>SMPSETPQAEVGPTGCPHRSGPHSAKGSLEKGSPEDKEAKEPLWIRPDAPSRCTWQLGRPASESPHHHTAPAKSPKILPDILKKIGDTPMVRINKIGKKFGLKCELLAKCEFFNAGGSVKDRISLRMIEDAERDGTLKPGDTIIEPTSGNTGIGLALAAAVRGYRCIIVMPEKMSSEKVDVLRALGAEIVRTPTNARFDSPESHVGVAWRLKNEIPNSHILDQYRNASNPLAHYDTTADEILQQCDGKLDMLVASVGTGGTITGIARKLKEKCPGCRIIGVDPEGSILAEPEELNQTEQTTYEVEGIGYDFIPTVLDRTVVDKWFKSNDEEAFTFARMLIAQEGLLCGGSAGSTVAVAVKAAQELQEGQRCVVILPDSVRNYMTKFLSDRWMLQKGFLKEEDLTEKKPWWWHLRVQELGLSAPLTVLPTITCGHTIEILREKGFDQAPVVDEAGVILGMVTLGNMLSSLLAGKVQPSDQVGKVIYKQFKQIRLTDTLGRLSHILEMDHFALVVHEQIQYHSTGKSSQRQMVFGVVTAIDLLNFVAAQERDQK[8x]

Cystathionine beta-synthase (CBS) is an essential metabolic enzyme across all domains of life for the production of glutathione, cysteine, and hydrogen sulfide. Human CBS adopts a unique multi-domain structure: an N-terminal haem binding domain (residues 38–74), a central PLP-dependent catalytic domain (CD, residues 75–382), and a C-terminal regulatory domain (RD, residues 411–551)5,11,12. The RD adopts the evolutionarily conserved Bateman module, consisting of two tandem CBS motifs (CBS-1 and CBS-2) and a surface-exposed loop (residues 516–525) extending from a CBS-2 motif. Here we show using cryo-electron microscopy that full-length human CBS in the basal and SAM-bound activated states polymerises as filaments mediated by a conserved regulatory domain loop.

We pursued the cryo-EM structure of full-length CBS initially using two constructs: one where an N-terminal His-tag was removed during purification (CBSFL) and one with a permanent C-terminal His-tag (CBSFL-CHis). Multiple maps were processed using both helical and single particle reconstruction to resolutions of between 3.9 and 3.0 Å. Both constructs resulted in maps with virtually identical conformations, and both were used for modelling. The domain-swapped dimer, previously observed in crystal structures, is the repeating unit, and helical formation is driven by inter-dimeric RD interactions, i.e., between the RDs of neighbouring subunits of the filament. Specifically, one RD each from two neighbouring CBS dimers interact in a butterfly-like dimeric arrangement, related by C2 symmetry, such that the loop 516–525 from an RD of one dimer forms a clasp around an RD of the neighbouring dimer. This packing arrangement, burying a total surface area of ~1550 Å2, is stabilised through two interfaces composed entirely of the RDs. The second interface involves inter-dimeric RD contacts, between the two neighbouring CBS-2 motifs. Here RD residues Leu419, Leu492, Met529, and Phe531 of one dimeric subunit form hydrophobic packing interactions with the equivalent residues of the neighbouring dimeric subunit. Altogether, the two sites of RD interactions demonstrate how loop 516–525 is the main driver of CBS oligomerisation. Though both full-length CBS constructs resulted in highly similar filament maps, one key difference was the observed protein degradation and the presence of slightly shorter oligomers of the CBSFL construct without a permanent His-tag.>[2x]TLSILVAHDLQRVIGFENQLPWHLPNDLKHVKKLSTGHTLVMGRKTFESIGKPLPNRRNVVLTSDTSFNVEGVDVIHSIEDIYQLPGHVFIFGGQTLFEEMIDKVDDMYITVIEGKFRGDTFFPPYTFEDWEVASSVEGKLDEKNTIPHTFLHLIRKLEHHHHHHHH

Dihydrofolate reductase (DHFR) is a critical enzyme in the recycling of folate cofactors that are essential for the synthesis of deoxythymidine monophosphate and several amino acids. Since inhibition of DHFR depletes the pool of available thymidine, it has proven to be an excellent drug target for rapidly proliferating bacteria, protozoa and cancer cells. Using high resolution structural information, we have developed a new class of antifolates characterized by a unique propargylic linker that shows activity against an expanded set of enzymes from important pathogens. Using a structure-based approach, a series of propargyl-linked antifolates were designed, synthesized and shown to possess highly potent antibacterial activity against both MRSA and S. pyogenes.

Interestingly, the structure-activity relationships observed in the biphenyl series did not directly translate to those analogs containing heterocyclic systems at ring C. Whereas the propargyl methyl and B-ring methoxy groups significantly impacted the activity of the biphenyl series, these substituents showed little effect in S. aureus DHFR across the heterocyclic series (compounds 24–28, 31, 36, 37). In order to understand the divergence between activity in the biphenyl and heterocyclic series, crystal structures of S. aureus DHFR bound to compounds 7 or 25 were determined. Comparison of the structures of S. aureus DHFR:NADPH:25 and S. aureus DHFR:NADPH:1 reveals a dramatic reorientation of the hydrophobic regions of the pyridyl series relative to the parent biphenyl analogs. In fact, a different enantiomer of pyridine 25 preferentially crystallizes relative to the enantiomer observed with 1. This new configuration forces a change in conformation for the nicotinamide ring of NADPH in order to maintain π-π stacking as well as a change in the conformation of Ile 50 that interacts with the proximal aryl ring. The stabilizing solvation of the pyridyl nitrogen at the opening of the active site drives the reorientation of compound 25 relative to compound 1. One consequence of this reorientation is decreased contact between the B- and C-rings and the active site residues, which is reflected in the slight attenuation in enzyme inhibition. In order to evaluate whether the compounds are bactericidal or bacteriostatic, we measured the minimum inhibitory and bactericidal concentrations (MBC) of compounds 24, 25 and TMP in strain Staphylococcus aureus subsp. aureus ATCC 44300. From these results, the MIC values match the MBC values for compounds 24 and 25, with both values equal to 0.078 µg/mL.>[2x]MIVDQFEEVLMKTSQLFPLPTATQSAQPTHVAPVPTVLPDTPIYETVGDSGSKTLWVVFVLMLIASAAFTALSWKIPVNRRLYHVITTIITLTAALSYFAMATGHGVALNKIVIRTQHDHVPDT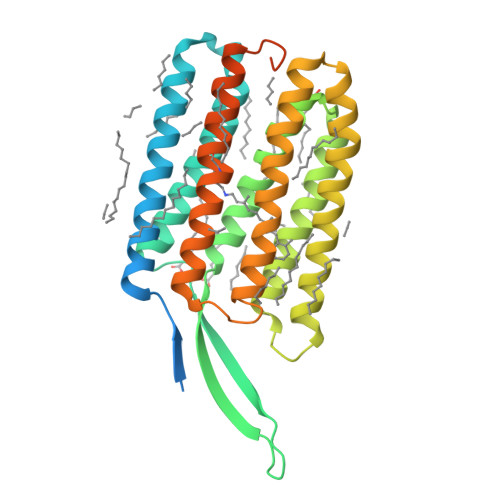YETVYRQVYYARYIDWAITTPLLLLDLGLLAGMSGAHIFMAIVADLIMVLTGLFAAFGSEGTPQKWGWYTIACIAYIFVVWHLVLNGGANARVKGEKLRSFFVAIGAYTLILWTAYPIVWGLADGARKIGVDGEIIAYAVLDVLAKGVFGAWLLVTHANLRESDVELNGFWANGLNREGAIRIGEDDGAGTHHHHHHHHH> FPTIPLSRLFDNAMLRAHRLHQLAFDTYQEFEEAYIPKEQKYSFLQNPQTSLCFSESIPTPSNREETQQKSNLELLRISLLLIQSWLEPVQFLRSVFANSLVYGASDSNVYDLLKDLEEGIQ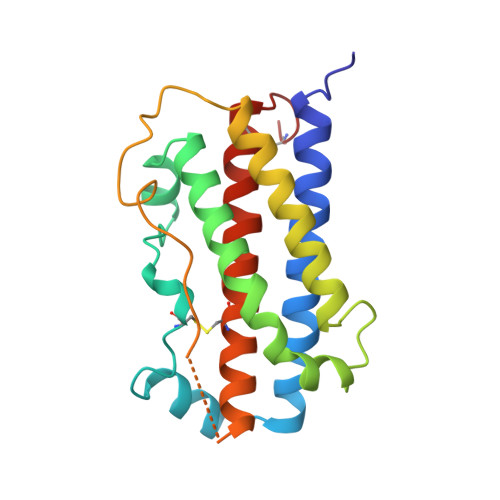TLMGRLEDGSPRTGQIFKQTYSKFDTNSHNDDALLKNYGLLYCFRKDMDKVETFLRIVQCRSVEGSCGF> MSLLLTIAKEYKRLCQDAKAAQMMTVGTVSNYTTFKKWTTSRKEKNPSLRMRWAMSSKFPIIANKRMLEEAQIPKEHNNVALWEDTEDVSKRDHVLASASCINYWNFCGPCVNNSEVIKEVYKSRFGRLERRKEIMWKELRFTLVDRQRRRVDTQPVEQRLRTGEIKDLQMWTLFEDEAPLASKFILDNYGLVKEMRSKFANKPLNKEVVAHMLEKQFNPESRFLPVFGAIRPERMELIHALGGETWIQEANTAGISNVDQRKNDIRAVCRKVCLAANASIMNAKSKLVEYIKSTSMRIGETERKL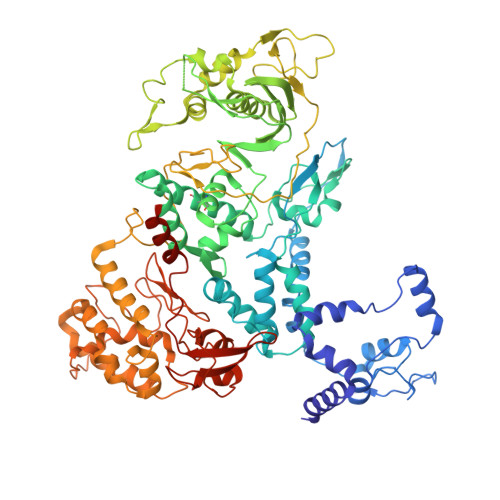EELILETDDVSPEVTLCKSALGGQLGKTLSFGPMLLKKISGSGVKVKDTVYIQGVRAVQFEYWSEQEEFYGEYKSATALFSRKERSLEWITIGGGINEDRKRLLAMCMIFCRDGDYFKDAPATITMADLSTKLGREIPYQYVMMNWIQKSEDNLEALLYSRGIVETNPGKMGSSMGIDGSKRAIKSLRAVTIQSGKIDMPESKEKIHLELSDNLEAFDSSGRIVATILDLPSDKKVTFQDVSFQHPDLAVLRDEKTAITKGYEALIKRLGTGDNDIPSLIAKKDYLSLYNLPEVKLMAPLIRPNRKGVYSRVARKLVSTQVTTGHYSLHELIKVLPFTYFAPKQGMFEGRLFFSNDSFVEPGVNNNVFSWSKADSSKIYCHGIAIRVPLVVGDEHMDTSLALLEGFSVCENDPRAPMVTRQDLIDVGFGQKVRLFVGQGSVRTFKRTASQRAASSDVNKNVKKIKMSNARENLYFQ>[8x]MVRFLDGHTPAYDLTYNDVFVVPGRSDVASRFDVDLSTVDGSGTTIPVVVANMTAVAGRRMAETVARRGGIVVLPQDLPITAVSETVDFVKSRDLVVDTPVTLSPEDSVSDANAL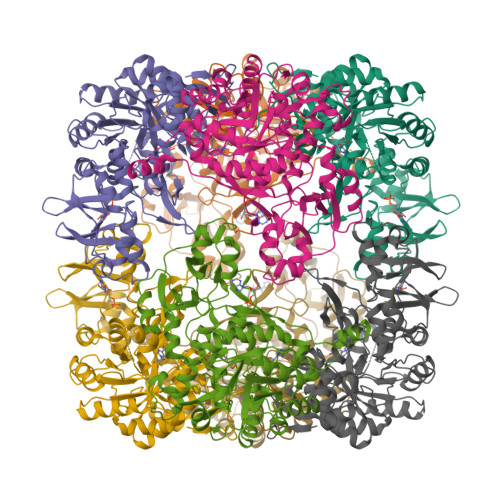LHKRAHGAAVVVFEGRPIGLVTEANCAGVDRFARVRDIALSDFVTAPVGTDPREVFDLLEHAPIDVAVMTAPDGTLAGVLTRTGAIRAGIYTPAVDAKGRLRIAAAVGINGDVGAKAQALAEAGADLLVIDTAHGHQAKMLDAIKAVASLDLGLPLVAGNVVSAEGTRDLIEAGASIVKVGVGPGAMCTTRMMTGVGRPQFSAVVECAAAARQLGGHVWADGGVRHPRDVALALAAGASNVMIGSWFAGTYESPGDLLFDRDDRPYKESYGMASKRAVAARTAGDSSFDRARKGLFEEGISTSRMSLDPARGGVEDLLDHITSGVRSTCTYVGAANLPELHEKVVLGVQSAAGFAEGHPLPAGWTAAAKEDLEHHHHHHHH>ETGQARLEKEYFDQHFGPFFRTEQLIIRAPLTDKHIYQPYPSGADVPFGPPLDIQILHQVLDLQIAIENITASYDNETVTLQDICLAPLSPYNTNCTILSVLNYFQNSHSVLDHKKGDDFFVYADYHTHFLYCVRAPASLNDTSLLHDPCLGTFGGPVFPWLVLGGYDDQNYNNATALVITFPVNNYYNDTE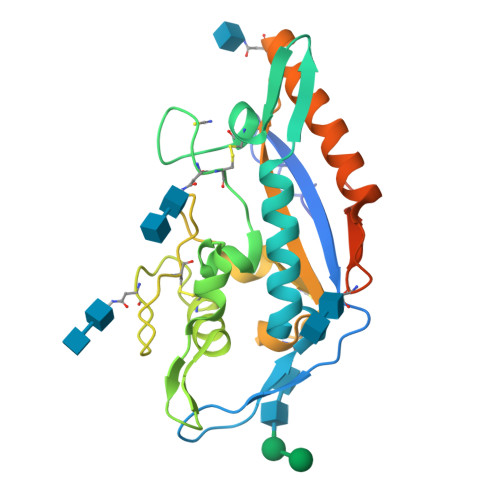KLQRAQAWEKEFINFVKNYKNPNLTISFTAERSIEDELNRESDTGTLEVLFQ[2x]[(1R,5S)-8-PHENETHYL-8-AZABICYCLO[3.2.1]OCTAN-3-YL] 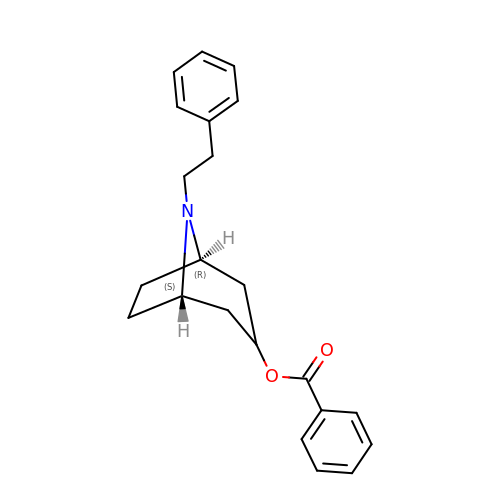BENZOATE | C22 H25 N O2 | ZVQCTZVWEBSXKK-AERCQKQUSA-N> MLRRSLVTFPWWNFQTEHRQRCVMMYGGSRAKNTHNANHRVFIKKYKRNAFPNRTRHHWAVSMTGVLGQRPRRMPWPYDLTSLIFNQPRQGSDKIGYVVGTSMLKTAVVAANHMVYYPKFNQRVSRTSRFFAHDEDLACVEGDLVHIKQCRKISKYKHYYVFSILEPNIEGRERLKLGLKAVPPPLFGYPVSRRIVKLNLTNAEGTKEKLAAVIQEHVQDAYRFAGPTPDQPRNRLTDSVTFDDANNMIAPNAPAT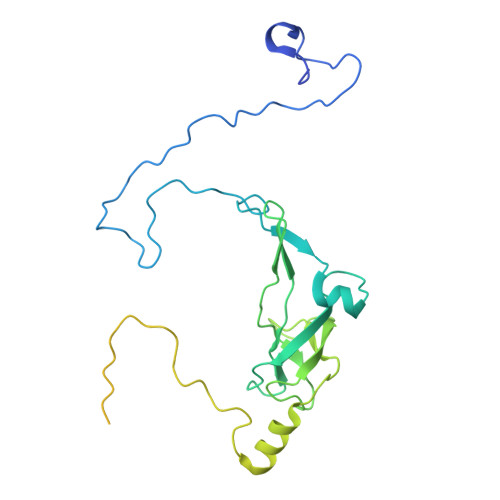PESLEGGESPSLLGDKEEYTEVEQDTRNKKGDEYWMNLQPKEKYDFKGFKKSP> AQPFAHLTINATDIPSGSHKVSLSSWYHDRGWAKISN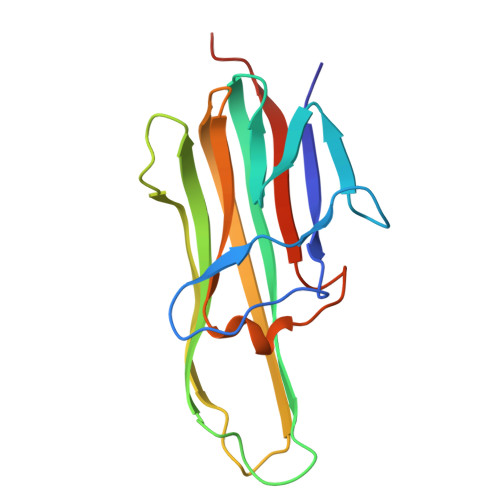MTFSNGKLIVNQDGFYYLYANICFRHHETSGDLATEYLQLMVYVTKTSIKIPSSHTLMKGGSTKYWSGNSEFHFYSINVGGFFKLRSGEEISIEVSNPSLLDPDQDATYFGAFKVRDIDHHHHHH> MKFKHQGLVADLLPNIRVMQGVGHFMFNYYSEGKKFPHRIYCIVTLLLLLLQYGMMAVNLMMESDDVDDLTANTITMLFFLHPIVKMIYFPVRSKIFYKTLAIWNNPNSHPLFAESNARFHALAITKMRRLLFCVAGATIFSVISWTGITFIEDSVKRITDPETNETTIIPIPRLMIRTFYPFNAMSGAGHVFALIYQFYYLVISMAVSNSLDVLFCSWLLFACEQLQHLKAIMKPLMELSATLDTVVPNSGELFKAGSADHLRESQGVQPSGNGDNVLDVDLRGIYSNRQDFTATFRPTAGTTFNGGVGPNGLTKKQEMLVRSAIKYWVERHKHVVRLVTAVGDAYGVALLLHMLTTTITLTLLAYQATKVNGVNVYAATVIGYLLYTLG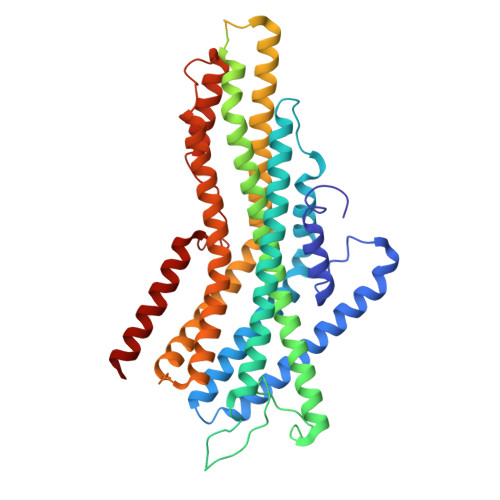QVFLFCIFGNRLIEESSSVMEAAYSCHWYDGSEEAKTFVQIVCQQCQKAMSISGAKFFTVSLDLFASVLGAVVTYFMVLVQLK>[2x]M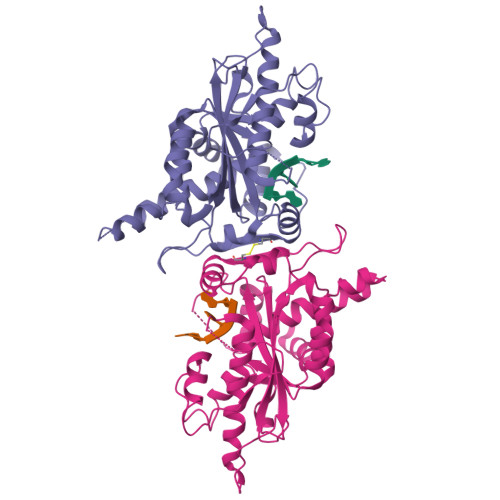EIIRSNFKSNLHKVYQAIEEADFFAIDGEFSGISDGPSVSALTNGFDTPEERYQKLKKHSMDFLLFQFGLCTFKYDYTDSKYITKSFNFYVFPKPFNRSSPDVKFVCQSSSIDFLASQGFDFNKVFRNGIPYLNQEEERQLREQYDEKRSQANGAGALSYVSPNTSKCPVTIPEDQKKFIDQVVEKIEDLLQSEENKNLDLEPCTGFQRKLIYQTLSWKYPKGIHVETLETEKKERYIVISKVDEEERKRREQQKHAKEQEELNDAVGFSRVIHAIANSGKLVIGHNMLLDVMHTVHQFYCPLPADLSEFKEMTTCVFPRLLDTKLMASTQPFKDIINNTSLAELEKRLKETPFNPPKVESAEGFPSYDTASEQLHEAGYDAYITGLCFISMANYLGSFLSPPKIHVSARSKLIEPFFNKLFLMRVMDI(2~{S})-2-[2-[2-[[2-methyl-3-oxidanyl-5-(phosphonooxymethyl)pyridin-4-yl]methylamino]ethylamino]-2-oxidanylidene-ethyl]-2-oxidanyl-butanedioic 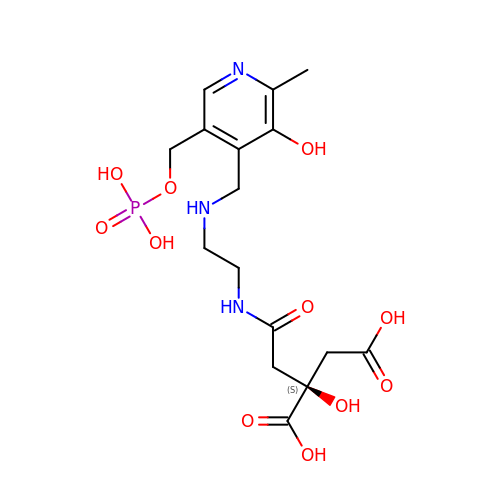acid | C16 H24 N3 O11 P | LHKUXYWSSPZJHQ-INIZCTEOSA-N> MS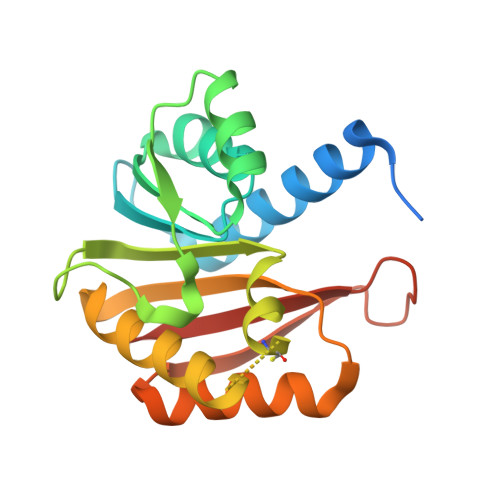RPEELAPPEIFYNDSEAHKYTGSTRVQHIQAKMTLRALELLNLQPCSFILDIGCGSGLSGEILTQEGDHVWCGLDISPSMLATGLSRELEGDLMLQDMGTGIPFRAGSFDAAISISAIQWLCNADTSYNDPKQRLMRFFNTLYAALKKGGKFVAQFYPKNDDQVDDILQSAKVAGFSGGLVVDDPESKKNKKYYLVLSSGHHHHHH>[2x]AIVLEEERYDLVEGQTLTVKCPFNIMKYANSQKAWQRLPDGKEPLT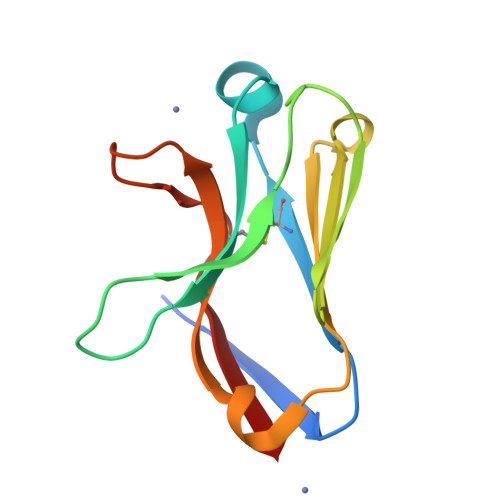LVVTQRPFTRPSEVHMGKFTLKHDPSEAMLQVQMTDLQVTDSGLYRCVIYHPPNDPVVLFHPVRLVVT>NTDLAIQGNGFFILKDGEKTFYTRAGAFGIDKEGTLVNPANGMRVQGWMAEEAEGFRIINTSGQTEDLNIPIGQKLDAKATTSVNYAANLDKRLPELPEGANRAQILESTWSTEFKVYDSFGEAHELQIDFARVPGEVNAWRATVNVDPTNADATATRVGIGTTDGVQNSFIVRFDNNGHLASVTDTAGNVTSPAGQVLVQISYNVVGANPDEAGAPTRHTFDVNLGEIGTSKNTITQFSDKSTTKAYEQDGYTLGYLENFRIDQSGIITGVYSNGVRQEIGQIAMAGFANQGGLEKAGQ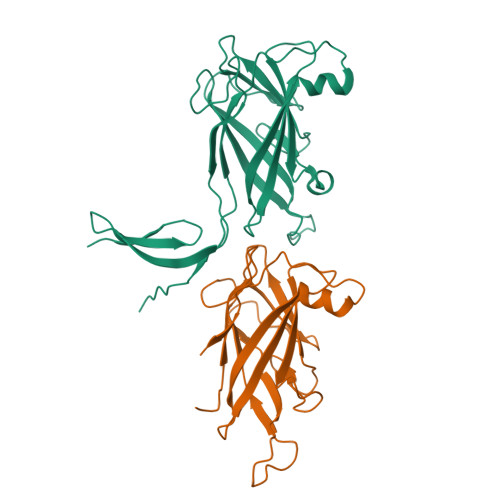NTYVQSNNSGIANVSTSGTVGKGYFIGGTLEMS[2x];>[2x]AKATTSVNYAANLDKRLPELPEGANRAQILESTWSTEFKVYDSFGEAHELQIDFARVPGEVNAWRATVNVDPTNADATATRVGIGTTDGVQNSFIVRFDNNGHLASVTDTAGNVTSPAGQVLVQISYNVVGANPDEAGAPTRHTFDVNLGEIGTSKNTITQFSDKSTTKAYEQDGYT> MFEKILLSNPSAENPSSLRPRKGIIIGLGQVGLACAYSMLIQDCFDELVLQDIASDKLEGEVMDFSHGMPFIPPTDIKAGTIANEGRNADIVIITAGVAQKEGESRLSLLERNIAIYKKILADVVKYCPEAIILVVTNPVDIMTYATLKITGFPSSRIIGSGTVLDTARFRTLLAKEMDIDPRSVHAYIIGEHGDSEVPVWSTANVGGMKLVPNTWADLPEDEKATLSGIFQKVQNAAYDIIKLKGYTSYAIGLATTDIVKAILNSQERILTVSGLMTGMYGIEDVCLSIPRVVSERGIIKTVNLTLSEDEEKLLQQSAKMLKEVFDKINYH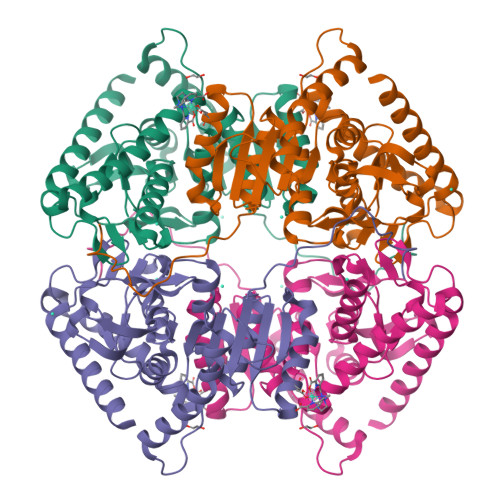HHHHH>MKILIVYTHPNPTSFNAEILKQVQTNLSKEHTVSTLDLYAEHFDPVLQFNETHKRRDLAKVAEMEKYRDLVTWADHLIFIFPIWWSGMPAILKGFIDRVFVADFAYSYKKVGLEGHLQGKSAWIITTHNTPSFAMPFVQDYGKVLKKQILKPCAISPVKLTELTSIEKISDDERQKLLHKVAQITRNILEHHH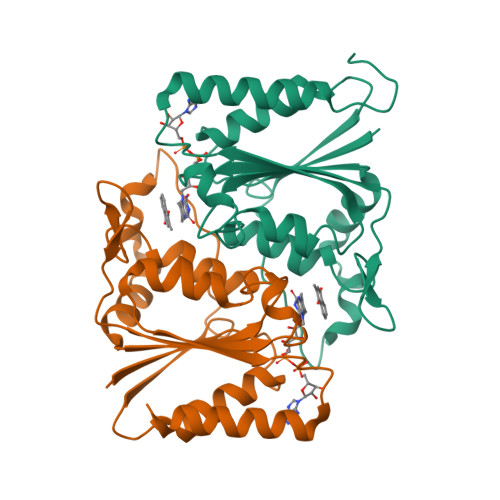HHH[4x]>[14x]TTTVGITLKDAVIMATERRVTMENFIMHKNGKKLFQIDTYTGMTIAGLVGDAQVLVRYMKAELELYRLQRRVNMPIEA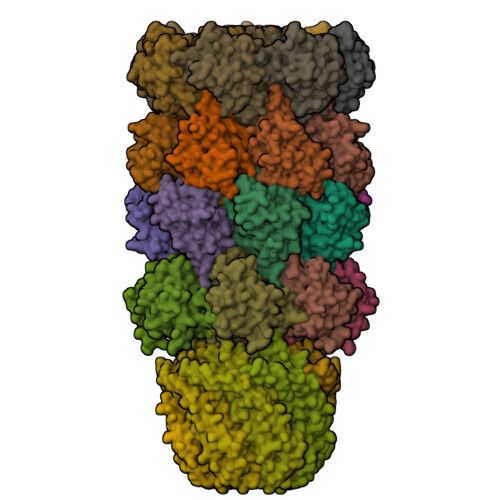VATLLSNMLNQVKYMPYMVQLLVGGIDTAPHVFSIDAAGGSVEDIYASTGSGSPFVYGVLESQYSEKMTVDEGVDLVIRAISAAKQRDSASGGMIDVAVITRKDGYVQLPTDQIESRIRKLGLIL;>AYDRAITVFSPDGRLFQVEYAREAVKKGSTALGMKFANGVLLISDKKVRSRLIEQNSIEKIQLIDDYVAAVTSGLVADARVLVDFARISAQQEKVTYGSLVNIENLVKRVADQMQQYTQYGGVRPYGVSLIFAGIDQIGPRLFDCDPAGTINEYKATAIGSGKDAVVSFLEREYKENLPEKEAVTLGIKALKSSLEEGEELKAPEIASITVGNKYRIYDQEEVKKFL[7x];>KRAALIQNLRDSYTETSSFAVIEEWAAGTLQEIEGIAKAAAEAHGVIRNSTYGRAQAEKSPEQLLGVLQRYQDLCHNVYCQAETIRTVIAIRIPEHKEEDNLGVAVQHAVLKIIDELEIKTLGSGEKSGSGGAPTPIGMYALREYLSARSTVEDKLLGSVDAESGKTKGGSQSPSLLLELRQIDADFMLKVELATTHLSTMVRAVINAYLLNWKKLIQPRTGTDHMFS[7x];>RAITVFSPDGRLFQVEYAREAVKKGSTALGMKFANGVLLISDKKVRSRLIEQNSIEAIQLIDDYVAAVTSGLVADARVLVDFARISAQQEKVTYGSLVNIENLVKRVADQMQQYTQYGGVRPYGVSLIFAGIDQIGPRLFDCDPAGTINEYKATAIGSGKDAVVSFLEREYKENLPEKEAVTLGIKALKSSLEEGEELKAPEIASITVGNKYRIYDQEEVKKFL[7x]>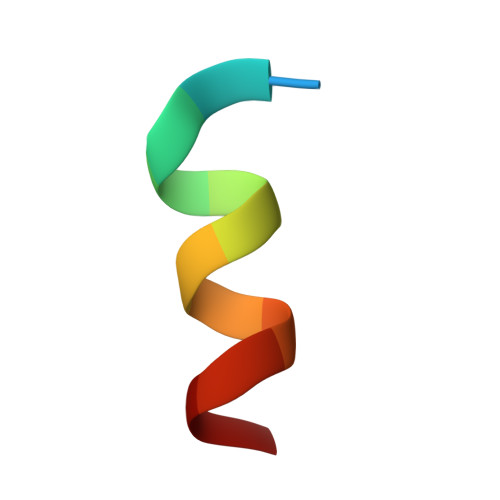 XLTFGEYWAQLAS> SGLKKFFPYSTNVLKGAAADIALPS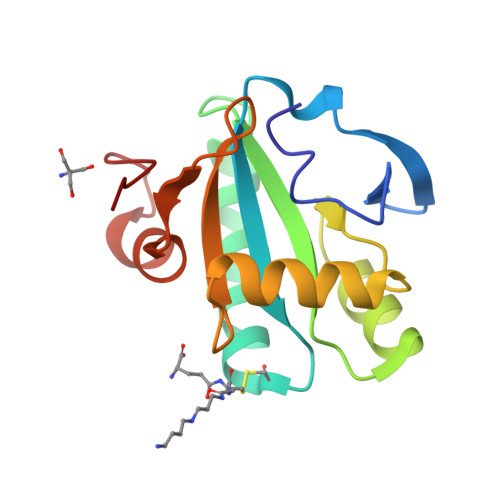LAGKTVFFYFSASWCPPSRAFTPQLIDFYKAHAEKKNFEVMLISWDESAEDFKDYYAKMPWLALPFEDRKGMEFLTTGFDVKSIPTLVGVEADSGNIITTQARTMVVKDPEAKDFPWPN>MEYKDTLLMPKTEFPMRGNLPNREPKMQEQWAEMNIYEKVQKRTEGRPLFVLHDGPPYANGDIHMGHALNKILKDFIVRYKSMSGFCAPYVPGWDTHGLPIETALTKNKKVNRKEMTVAEFRKLCEQYAWEQVNGQREQFKRLGVRGDWDNPYVTLQPQYEAQQIKVFGDMAKKGYIYKGLKPVYWSPSSESALAEAEIEYYDKRSASIYVAFNVKDGKGVLEQDEKFIIWTTTPWTMPANQGIAVNPELQYSVVEADGAKYVVATELIETVAKEIEWADYKTLRTVKGSELERVVAEHPIYKRDSLVVLGDHVTTDAGTGCVHTAPGHGEDDFIVGQKYGLEVLCPVDSKGHMTNEAPGFEGLFYDKANKPITDKLEEEGALLKLSFITHSYPHDWRTKKPTIFRATAQWFASIKDFREDLLKAVEKTKWVPTWGETRLYNMVRDRGDWCISRQRAWGVPIPVFYAENEEPIITDETIEHVSNLFREHGSNVWFEREAKDLLPEGFTHEGSPNGRFTKETDIMDVWFDSGSSHQAVLEEREDLQRPADLYLEGSDQYRGWFNSSLSTSVAVTGEAPYKGVLSHGFALDGEGRKMSKSLGNVVIPEKVMKQLGADILRLWVASVDYQADVRVSDNILKQVAEVYRKIRNTFRFLLGNLADFNPTTDAVAVEDLREVDRYMLVKLNKLIDKVKKSYDSYEFSSIYHAVHNFCTIDMSSFYLDFAKDVLYIEAENNVERRSIQTVLYETLLSLTKLVSPILSHTADEVWVHIPNVTEESVQLVDMPEVQEIEGADQLVEKWDAFMELRDEVLKALEQARNEKVIGKSLEAKLTLYPTADTKELLASISENVGQLFIVSDLEVAEGEAPAEAQKFSYASIVVSKAEGEKCERCWVVSPTVGEDQDHPTLCTRCADVVKNHYVQQ[2x]

Mupirocin, a clinically used natural antibiotic, inhibits isoleucyl-tRNA synthetase (IleRS), an enzyme that links isoleucine to its tRNAIle for protein synthesis. Two IleRSs, mupirocin-sensitive IleRS1 and resistant IleRS2, coexist in bacteria. Specifically, type 1 proteins (IleRS1) are strongly inhibited by mupirocin (Ki in low nanomolar range), while IleRS2, which are homologous to IleRSs from the eukaryote cytosol, exhibit resistance to mupirocin concentrations that are about three orders of magnitude higher. AARSs catalyze the formation of AA-tRNA in two steps within the same active site. The amino acid is first activated by ATP to form an aminoacyl-adenylate (AA-AMP) intermediate, followed by the transfer of the aminoacyl moiety to the tRNA.

Therefore, to deepen our understanding of mupirocin resistance in general and to infer the mechanism of hyper-resistance, we determined the crystal structures of wild-type PmIleRS1 (sensitive) and PmIleRS2 (resistant), both of which carry the canonical HXGH motif and are amenable in mupirocin-bound form when the inhibitor is supplied at sufficiently high concentrations. To alleviate this problem, we solved the structures of IleRS1 (sensitive) and IleRS2 (resistant) from P. megaterium bound to mupirocin only. The overall structures of mupirocin-bound PmIleRS1 and PmIleRS2 overlap well with those determined in complex with Ile-AMS. The binding of mupirocin to both (sensitive and resistant) enzymes is similar as described; however, we are able to reveal distinct interactions. We observe the backbone of Pro56 and the side chain of Asn70 forming interactions with O13 and O7 atoms of mupirocin, respectively, in PmIleRS1, which are absent in PmIleRS2. Furthermore, stacking interactions of Phe586 and the unsaturated C2-C3 bond of the monic acid A part contributes to the affinity in IleRS1, while the analogous His582 is reoriented in PmIleRS2. Finally, we found that the carboxylate oxygen of the nonanoic acid part of mupirocin establishes an H-bond with the backbone NH of K597 from the KMSKS loop only in PmIleRS1. No such ligand-dependent rearrangements in the HXGH motif are observed in PmIleRS1.>GPKPKNTKENLSKSSWRQEWLANLKLISVSLVDEFPSELSDSDRQIINEKMQLLKDIFANNLKSAISNNFRESDIIILKGEIEDYPMSSEIK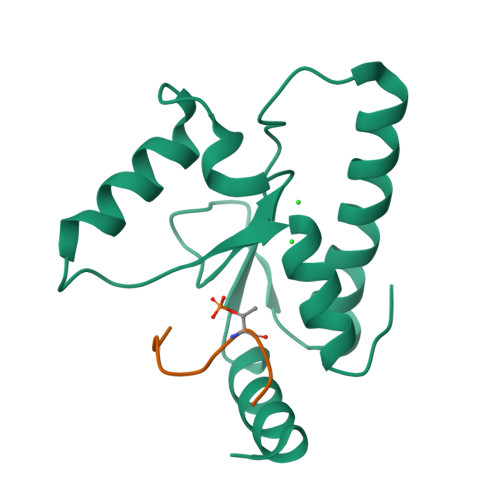IYYNELQNKPDAKKARFWSFMKTQRFVSNMGFDIQ[7x];>[7x]LSTELSTEPPSS>[2x]LA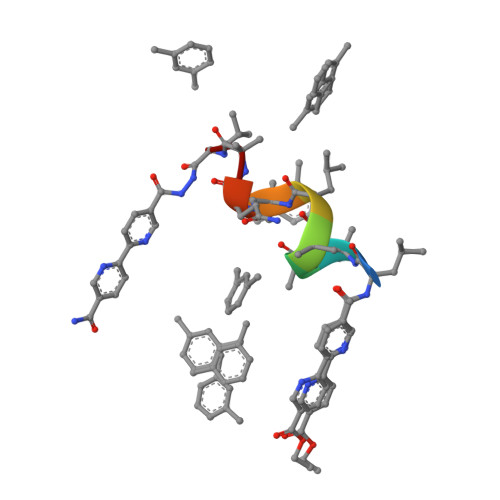AALAQAL2-[(4-amino-3-methylpyridin-2-yl)methyl]-1,2,3,4-tetrahydroisoquinolin-8-amine 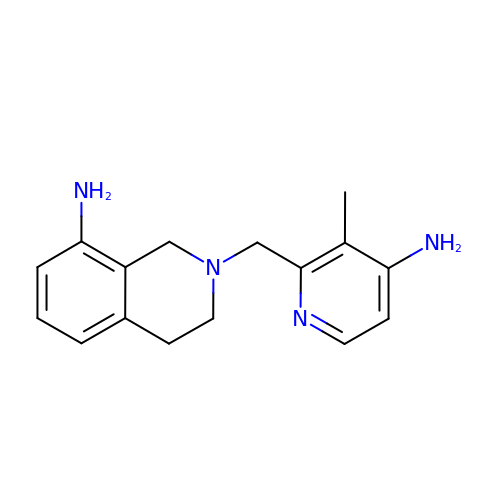| C16 H20 N4 | HNIXXQJEZDAUFJ-UHFFFAOYSA-N> MELKHSISDYTEAEFLQLVTTICNADTSSEEELVKLVTHFEEMTEHPSGSDLIYFPKEGDDDSPSGIVN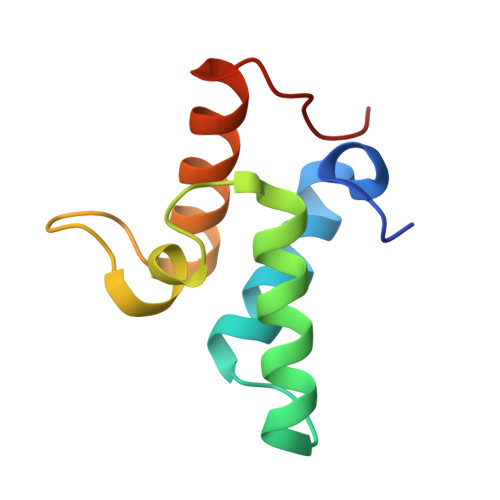TVKQWRAANGKSGFKQG>MVSLMFFSSASPLCSSPSKIPKASLDFEMKKLGGSTKLVRNVNLEKLKNNYLFPEINRRELEHIEKHPNVQLISLGTGDTTEPIPEQITSHMSNFAHGLSTVEGYRGYGLEQGNKTLRKAIAETFYRDLHVKSNEVFVSDGAQSDISRLQLLLGSNVTIAVQDPTFPAYIDSSVIIGQTGHFHEKTKKYQNVVYMPCGPNNSFFPDLAMTPRTDVIFFCSPNNPTGYVASRKQLHQLVDFAKTNGSIIIFDSAYAAFIEDGSPRSIYEIPGAREVAIEVSSFSKFA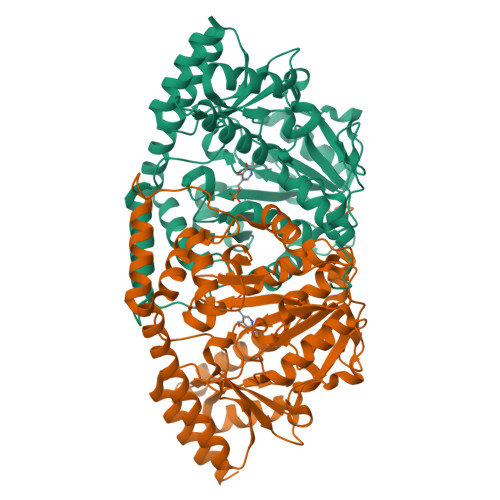GFTGVRLGWSIIPDELLYSNGFPIINDFHRIVTTSFNGASNIAQAGGLACLSSGGLKEIRSVNNYYKENRKILMDTLVSLGLKVYGGVNAPYLWVHFKGSKSWDVFNEILENTHIITVPGSGFGPGGEEYLRISGFGRRDHIVEASKRLQNFFNTRTKHFTYLSSTSNTN[2x]> MGSSHHHHHHSSGRENLYFQGHMQKVVLATGNVGKVRELASLLSDFGLDIVAQTDLGVDSAEETGLTFIENAILKARHAAKVTALPAIADDSGLAVDVLGGAPGIYSARYSGEDATDQKNLQKLLETMKDVPDDQRQARFHCVLVYLRHAEDPTPLVCHGSWPGVITREPAGTGGFGYDPIFFVPSEGKTAAELTREEKSAISHRGQALKLLLDALRNGG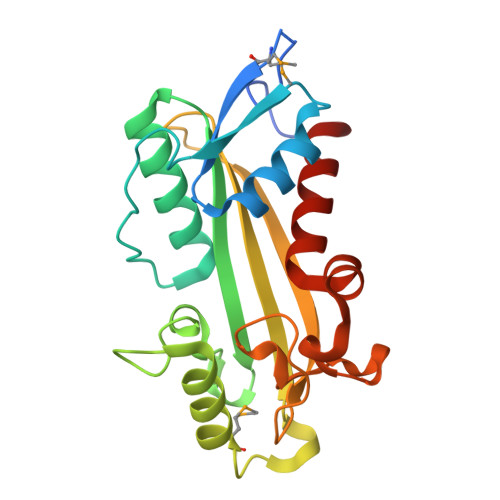S>MEMILEEKDASDWIYRGEGGANLVLAYAGSSPLFVGKVIRIQKARRNDKAIKNSNGVVSVLTSDEQHLWRENNELISSPNKEVLEQRYVQNVIIPLLGPKHVDAGVRVSVSKEFLECVDKKVTKQRPLWRVNAANVDTSHDSALILNDHSLFSQGITSGGDCISVEIKPKCGFLPTSRFIGKENMLKTSVSRFKMHQLLKLEYIEISEESEYDPLDLFSGSKERVLEAIKALYSTPQNNFRVFL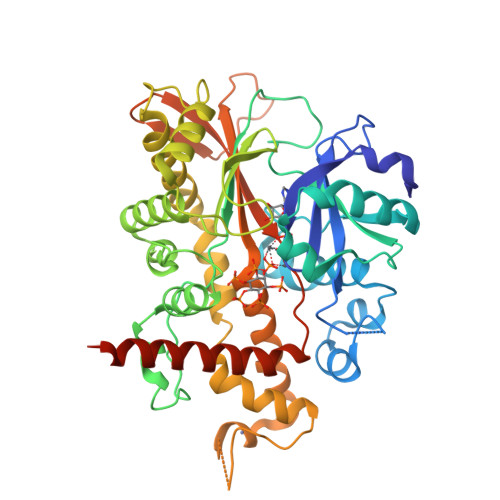NGSLILGGSGESTGRTSPEIGYAFEDALKGFIQSEDGHRTECFLQLVSDAVYGSGVLDRLLEIQKLDKLDIEGAIHCYYDIINQPCPICKEGRPLEAELSLHALPLDESLKIVKEYLIAATAKDCSIMISFQSRNAWDSEPSGDYVSLKPTNQTFDYKVHFIDLSLKPLKRMESYYKLDKKIISFYNRKQKAENTAEQIGNSKPSHS[2x]>GGGUCGCCGAUGUGCAGCAUAGGUAGGAGACACUACACAGGUACCCGCGCUAGCGGGCCACCGAGUCAACAGUGAAAUACUACCCGUCGGUGACCC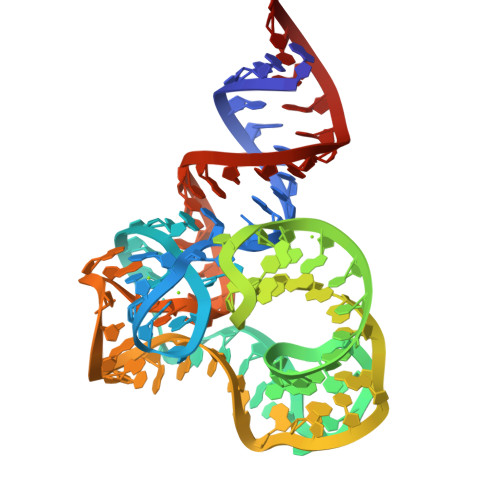[2x]> RIIYDRKFLMEC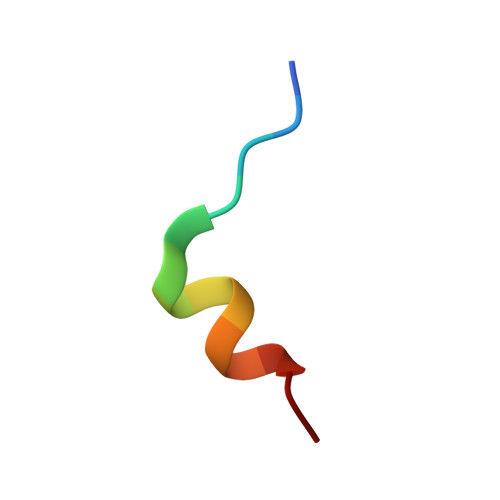RN>[2x]MAVFEQNKRPKISLIGSGMIGGTMAYLCAL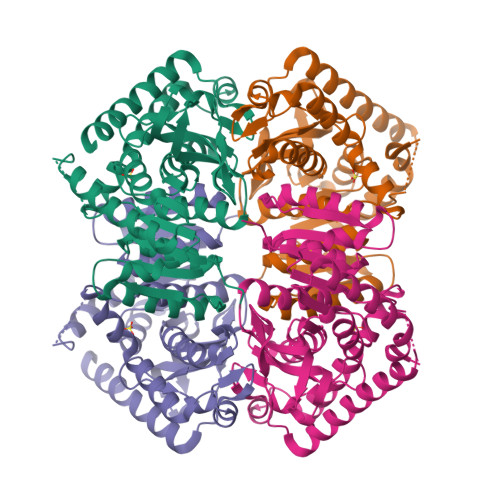KELGDVVLFDVVKNMPQGKALDLSHSTSVADTNVKVTGTNSYEDIKGSDVVIITAGLTKVPGKSDKEWSRDDLLPINAKIMKEVGENIKKYCPNAFVICITNPLDVMVKVLQEASGLPHNKVCGMAGVLDSSRFRYFIAEKLNVSPRDVQAMVIGAHGDNMVPLPRYVTVNGIPLQEFIKKGWITQEEIDEIVERTRNAGGEIVNLLGTGSAYFAPAASAIAMAEAYLKDQKRVLPCSCYLEGQYGVKDLYVGVPVVIGGNGVEKVIELELTPEEKEMFDKSIEEVRELVKALEALDAPA>[2x]MVFYMTALFPYIAFENSKEALAYYEEVFGATDVKRLE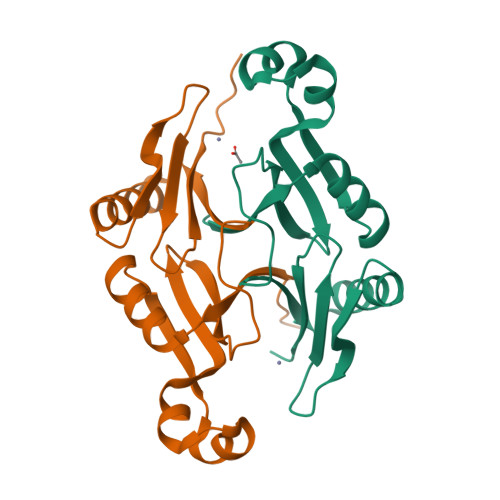VGEEQASHFGMTKEEAQEATMHAEFEVLGVKVLCSDSFGRADKINNGISLLIDYDVNNKEDADKVEAFYEQIKDHSSIEIELPFADQFWGGKMGVFTDKYGVRWMLHGQDYTAIQQ> GPGSELPQMVQQLNSPDQQELQSALRKLSQIASGGNEQIQKLIEAGALSPLVKLL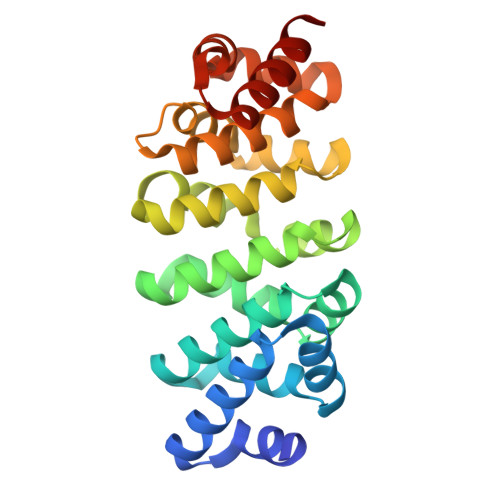DDASEEVIQEAVWAIANIASGNNEQIQKLIEAGALSPLVKLLDDASEEVIQEAVWAIANIASGNNEQIQKLIEAGALSPLVKLLDDASEEVIQEAVWAIANIASGNNEQIQKLIEAGALSPLVKLLDDASEEVIQEAVWAIANIASGNNEQIQKLEEAGAEPALEKLQSSPNEEVQKNAQAALEALNS> ADDIVLKAKNGDTKFP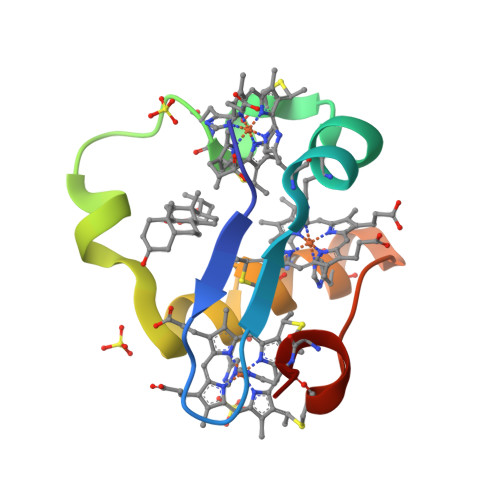HKAHQKAVPDCKKCHEKGPGKIEGFGKEMAHGKGCKGCHEEMKKGPTKCGECHKK> 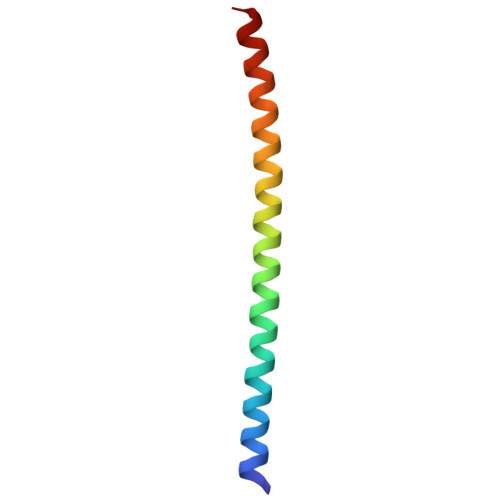STENLYFQSNADSVQNHTFEVENNTINGLELTEEQVHILYAMVLQTHADVQLLKEQQ> MKDLIIPPLDWTQDMGTPKREGAPVHLTIDGVEVTVPAGTSVLRAAAEAGISIPKLCATDNVEPVGSCRLCMVEIEGMRGTPTSCTTPVAPGMRVHTQTPQLQKLRRGVMELYISDHPLDCLTCAANGDCELQDMAGAVGLREVRYQAKDTHFARRDATGPNPRYIPKDNSNPYFSYDPAKCIVCMRCVRACEEVQGTFALTVMGRGFDARISPAAPDFLSSDCVSCGACVQACPTATLVEKSVERIGTPERKVVTTCAYCGVGCSFEAHMLGDQLVRMVPWKGGAANRGHSCVKGRFAYGYATHQDRILKPMIRDKITDPWREVNWTEALDFTATRLRALRDSHGADALGVITSSRCTNEETYLVQKLARAVFGTNNTDTCARVCHSPTGYGLKQTFGTSAGTQDFDSVEETDLALVIGANPTDGHPVFASRLRKRLRAGAKLIVVDPRRIDLLNTPHRGEAWHLQLKPGTNVAVMTAMAHVIVTEQIFDKRFIGDRCDWDEWADYAEFVANPEYAPEAVESLTGVPAGLLRQAARAYAAAPNAAIYYGLGVTEHSQGSTTVIAIANLAMMTGNIGRPGVGVNPLRGQNNVQGSCDMGSFPHEFPGYRHVSDDATRGLFERTWGVTLSSEPGLRIPNMLDAAVEGRFKALYVQGEDILQSDPDTRHVSAGLAAMDLVIVHDLFLNETANYAHVFLPGSTFLEKDGTFTNAERRINRVRRVMAPKAGFADWEVTQMLANALGAGWHYTHPSEIMAEIAATTPGFAAVTYEMLDARGSVQWPCNEKAPEGSPIMHVEGFVRGKGRFIRTAYLPTDEKTGPRFPLLLTTGRILSQYNVGAQTRRTENTVWHGEDRLEIHPTDAETRGIRDGDWVRLASRA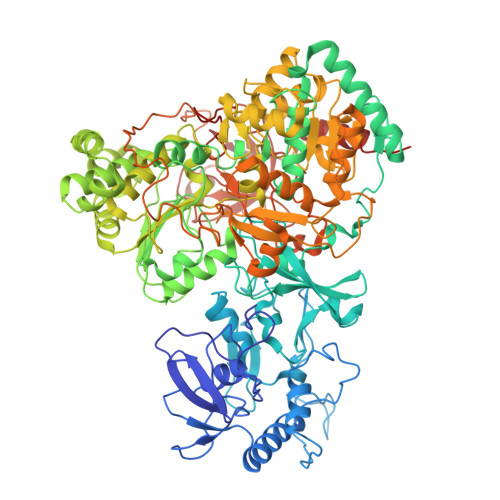GETTLRATVTDRVSPGVVYTTFHHPDTQANVVTTDTSDWATNCPEYKVTAVQVAASNGPSDWQQDYAAQAAAARRIEAAE3-methyl-5-(2-phenoxyphenyl)pyridin-2(1H)-one | C18 H15 N O2 | 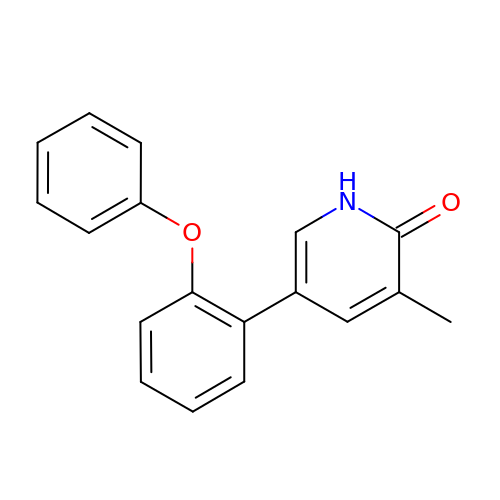ZQYOXBNCDYICCV-UHFFFAOYSA-N>[4x]GPGVDHC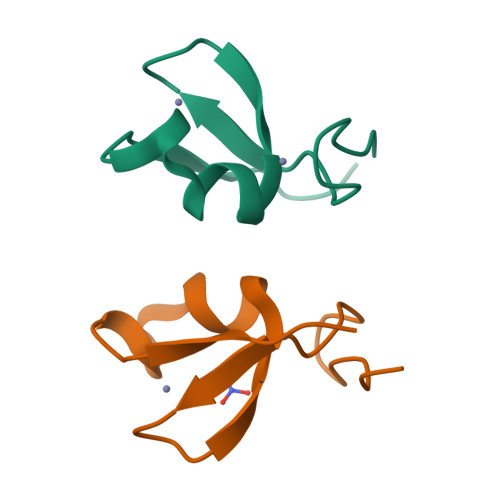ARHGEKLLLFCQEDSKVICWLCERSQEHRGHHTFLMEEVAQEYHVKLQTALEMLRQKGGDPYMRELISELEHRLQGSMMDLLQGVDGIIKRIEN> MDKNSNGKLIALAVGGAVLMGALFFSVSFLTGYIPAPNHSAILTPLRSFMGWFLLIFCASIIIMGLGKMSSAISDKWFLSFPLSIFVIVMVMFLSLRVYWEKGRTTTVDGKYIRTTAELKEFLNKPAATSDVPPAPAGFDFDAAKKLVDVRCNKCHTLDSVADLFRTKYKKTGQVNLIVKRMQGFPG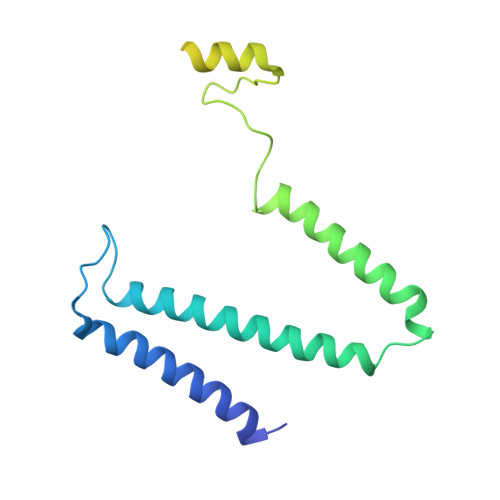SGISDDDAKTIGIWLHEKF> MEAVLYSTFRNHLKDYMKKVNDE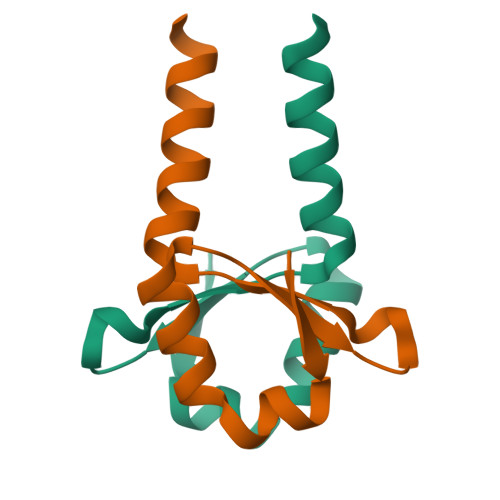FEPLTVVNKNPDEDIVVLSKSEWDSIQETLRIAQNK>[5x]GSHMGGVEVLEVKTGVDSITEVECFLTPEMGDPDEHLRGFSKSISISDTFESDSPNRDMLPCYSVARIPLPNLNEDLTCGNILMWEAVTLKTEVIGVTSLMNVHSNGQATHDNGAGKPVQGTSFHFFSVGGEALELQGVLFN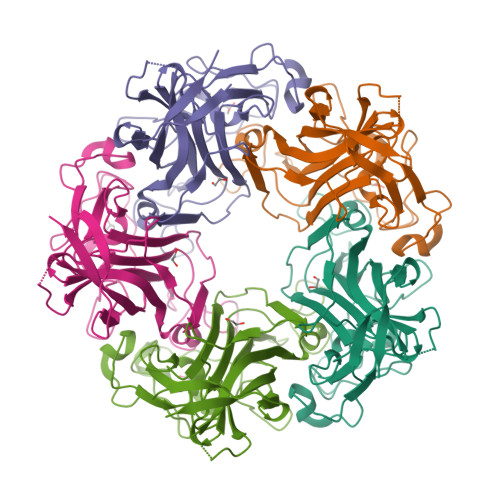YRTKYPDGTIFPKNATVQSQVMNTEHKAYLDKNKAYPVECWVPDPTRNENTRYFGTLTGGEQVPPVLHITNTATTVLLDEFGVGPLCKGDNLYLSAVDVCGMFTNRSGSQQWRGLSRYFKVQLRKRRVKN>GANRTLIVTTILEEPYVMYRKSDKPLYGNDRFEGYCLDLLKELSNILGFLYDVKLVPDGKYGAQNDKGEWNGMVKELIDHRADLAVAPLTITYVREKVIDFSKPFMTLGISILYRKGTPIDSADDLAKQTKIEYGAVRDGSTMTFFKKSKISTYEKMWAFMSSRQQSALVKNSDEG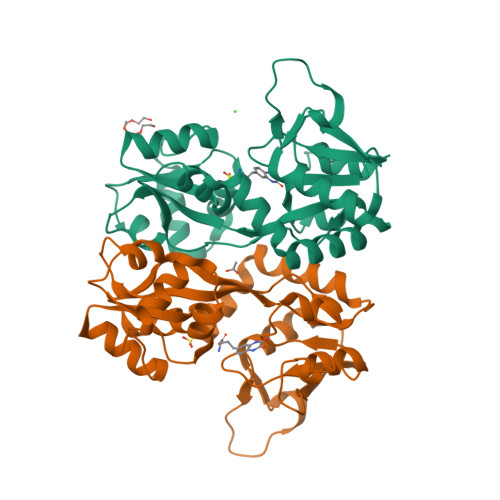IQRVLTTDYALLMESTSIEYVTQRNCNLTQIGGLIDSKGYGVGTPIGSPYRDKITIAILQLQEEGKLHMMKEKWWRGNGCP[3x]>[2x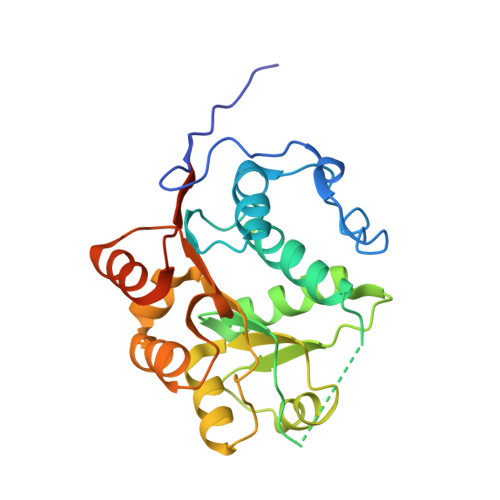]FDKYDSIPVSVTGPDYSATNVIENFDELKLDPTIRNNILLASYQRPTPIQKNAIPAILEHRDIMACAQTGSGKTAAFLIPIINHLVCQDLNQQRYSKTAYPKCLILAPTRELAIQILSESQKFSLNTPLRSCVVYGGADTHSQIREVQMGCHLLVATPGRLVDFIEKNKISLEFCKYIVLDEADRMLDMGFEPQIRKIIEESNMPSGINRQTLMFSATFPKEIQKLAADFLYNYIFMTVGRVGSTSDSIKQEI>[4x]GSHMVGDNKLDDKNIDKEKESSYRFPVIAMKVKKGILSDYLSLNGDVDTKVKADIFPDAVGKITSLRIKLGAYVQKGQIVATLDPSRPGSVYLKSPVRAPISGYILNITKKIGETVNPQSNIAVVGRIDTKQILTYVSEKYISNIKVGNDAIIEVGAYSNEKFKAKVSEISPILDSKSRTIEVYLTPIGSNLDKLIIGMFSKIKLITKRFKDVIKISREAVVEREGKKFVFKVDLESKSVQMLPITVLFEIDNIVALSGEVEENDLIVVEGMSALSNGSLINLVDTKEGLSAESNI

Periplasmic adaptor proteins are essential components of bacterial tripartite multidrug efflux pumps. BesA shows the archetypal linear, flexible, multi-domain architecture evident among proteobacteria and retains the lipoyl, β-barrel and membrane-proximal domains that interact with the periplasmic domains of the inner membrane transporter. However, it lacks the α-hairpin domain shown to establish extensive coiled-coil interactions with the periplasmic entrance helices of the outer membrane-anchored TolC exit duct. The adaptor multidomain structure is conserved throughout proteobacteria, but primary sequence comparison in the spirochete Borrelia burgdorferi suggested that a tripartite MDR pump, BesABC, included an adaptor that appeared to lack an α-hairpin.

The crystal structure of the complete BesA protein was solved by SAD in three space groups, P212121 (2.35 Å resolution), P21 (2.5 Å) and C2 (2.6 Å), in which either a monomer (C2) or four intertwined head-to-tail monomers (P21 and P212121) are present in the asymmetric unit. Given the protein is membrane localised by an N-terminal lipidation, this head-to-tail arrangement, also seen in the isolated CusB structure, cannot be physiologically relevant. The BesA monomer shows the archetypal, multidomain adaptor topology, with the MP, β-barrel, and lipoyl domains in linear arrangement (coloured orange, yellow and green, respectively). However, the expected final α-hairpin domain is completely absent, confirming what was predicted from sequence analysis, leaving only a nine residue loop (Pro106 to Leu114, blue in Fig. 1B) linking the two halves of the lipoyl domain. Density for this loop is visible only in the C2 monomer where it is stabilised by the loop of a neighbouring monomer in the crystal lattice, but high B-factors here and poorly defined density for the P212121 or P21 monomers indicate the small loop is highly flexible. In both the data-based assembly model of AcrAB-TolC and the in vitro co-crystal structure of an adaptor-transporter (CusBA) subcomplex tripartite pump assembly is facilitated by the flexibility of the adaptor’s serially-linked domains, which was confirmed by MD analysis of the closely related MexA. This ‘hinge’ flexibility at the inter-domain linkers is also evident in the BesA variant space groups which show movement of the lipoyl domain, relative to the other domains.> MKKYHISMINI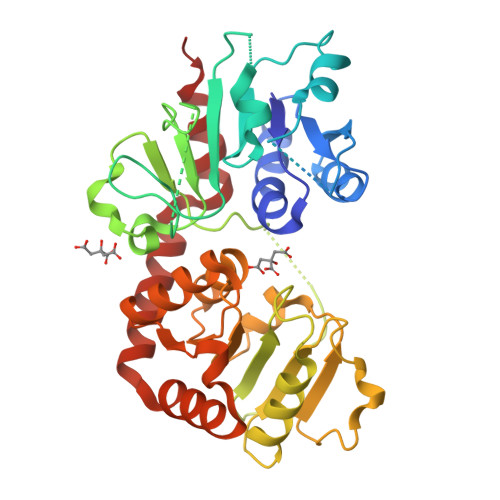PAYGHVNPTLALVEKLCEKGHRVTYATTEEFAPAVQQAGGEALIYHTSLNIDPKQIREMMEKNDAPLSLLKESLSILPQLEELYKDDQPDLIIYDFVALAGKLFAEKLNVPVIKLCSSYAQNESFQLGNEDMLKKIREAEAEFKAYLEQEKLPAVSFEQLAVPEALNIVFMPKSFQIQHETFDDRFCFVGPSLGERKEKESLLIDKDDRPLMLISLGTAFNAWPEFYKMCIKAFRDSSWQVIMSVGKTIDPESLEDIPANFTIRQSVPQLEVLEKADLFISHGGMNSTMEAMNAGVPLVVIPQMYEQELTANRVDELGLGVYLPKEEVTVSSLQEAVQAVSSDQELLSRVKNMQKDVKEAGGAERAAAEIEAFMKK> AEQAQPKTPENSSTEQPTVKATQTTEQAITEKQQQVTEKQAIVDQKQQVADTAKKEKDAIDQSVKDQQAVVDQNKDALDQSQQAVTDQQAVVDEAKKVVDEATPSAIEKAKEQVATDTQAVDEQQKVVDQAQTDVNQQQAVVDEKAKETNAAKVQNEKDQQAVTAAKQEQAKLEELAKNAEAEKVKAEKEQAAKEAELANKQKEEAKAKDQKTKDDQAVADQQTVVTTSQEKVTDAKADTAAKQADLTAKENALKDKQAATKQAQNTLDNSKEELKGHKGINLPPKFSADYDTKLSAEEIATLEKTALEMNKNFPTSKEDEKNKDVMWDIQHLSADQKKELS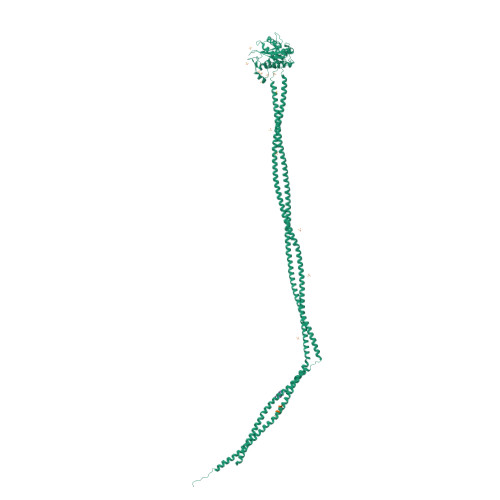VYTTELLNDVRKKLGLSQLSVSDQSIKFAWDIAKYSDTGEYMHDVIAINKAAKENGFKEYPGMNYYENLGGGYYETENGKVSKYTLQESIRKMLVNMLFDDGRLGYSHLHSLLQDGKTALGVSLSGEKNSISPKIHIISYGKEKLEDSSQYQNGEVASMKSKEELQQEIASNQEKLATAQQAESDAQQARSASQQALNTAKTTQATAEKELSVHKATLANLQAVATKSTTNYEEKVRQTATAEKSLQQTKDQLATINELIQNRAAVLEKAKTNVAEAQAIEQTSAKVLKEKQEAQKAEENTLNSLKEVLDLAKENLNQKQVALKTSTRSLSRLENAQPTYEKALNELNKAEAAVVQAQEAYENSMKSLEELKEQQAVATLAYAQAQEDLSNAKLELQQYQGVLRDLEAQQAEQRRQEALQEQVAKEQQRLEREAKQNQTLVASAT;>AAAAAAAAA[2x]> SSSYTEADPAILSRRQKQIDYGKNTAAYERYVEMVPKDERTRDHPRTP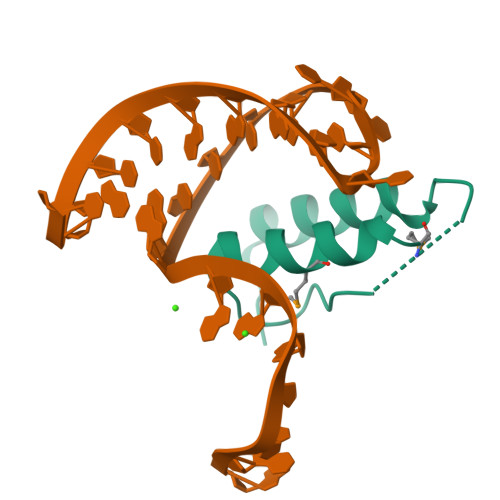NKYGKYSRRAFDGMVKIWRKSMHIYDPPTQARDTAKDSNSDSDSD> EPLDDYVNTQGASLFSVTKKQLGAGSIEECAAKCEEDEEFTCRAFQYHSKEQQCVIMAENRKSSIIIRMRDVVLFEKKVYLSECKTGNGKNYRGTMSKTKNGITCQKWSSTSPHRPRFSPATHPSEGLEENYCRNPDNDPQGPWCYTTDPEKRYDYCDILECEEECMHCSGENYDGKISKTMSGLECQAWDSQSPHAHGYIPSKFPNKNLKKNYCRNPDRELRPWCFTTDPNKRWELCDIPRCTTPPPSSGPTYQCLKGTGENYRGNVAVTVSGHTCQHWSAQTPHTHNRTPENFPCKNLDENYCRNPDGKRAPWCHTTNSQVRWEYCKIPSCDSSPVSTEQLAPTAPPELTPVVQDCYHGDGQSYRGTSSTTTTGKKCQSWSSMTPHRHQKTPE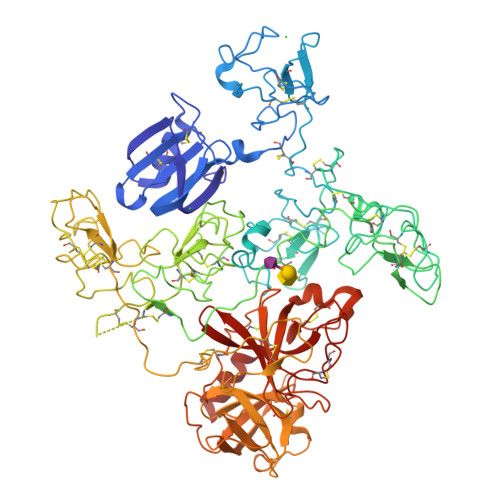NYPNAGLTMNYCRNPDADKGPWCFTTDPSVRWEYCNLKKCSGTEASVVAPPPVVLLPDVETPSEEDCMFGNGKGYRGKRATTVTGTPCQDWAAQEPHRHSIFTPETNPRAGLEKNYCRNPDGDVGGPWCYTTNPRKLYDYCDVPQCAAPSFDCGKPQVEPKKCPGRVVGGCVAHPHSWPWQVSLRTRFGMHFCGGTLISPEWVLTAAHCLEKSPRPSSYKVILGAHQEVNLEPHVQEIEVSRLFLEPTRKDIALLKLSSPAVITDKVIPACLPSPNYVVADRTECFITGWGETQGTFGAGLLKEAQLPVIENKVCNRYEFLNGRVQSTELCAGHLAGGTDSCQGDSGGPLVCFEKDKYILQGVTSWGLGCARPNKPGVYVRVSRFVTWIEGVMRNN> MLEEALAAIQNARDLEELKALKARYLGKKGLLTQEMKGLSALPLEERRKRGQELNAIKAALEAALEAREKALEEAALKEALERERVDVSLPGASLFSGGLHPITLMERELVEIFRALGYQAVEGPEVESEFFNFDALNIPEHHPARDMWDTFWLTGEGFRLEGPLGEEVEGRLLLRTHTSPMQVRYMVAHTPPFRIVVPGRVFRFEQTDATHEAVFHQLEGLVVGEGIAMAHLKGAIYELAQAL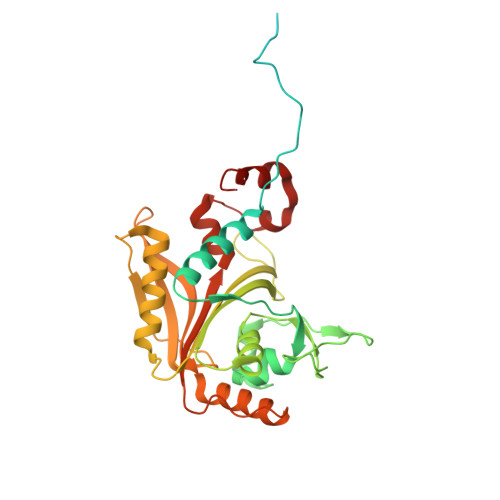FGPDSKVRFQPVYFPFVEPGAQFAVWWPEGGKWLELGGAGMVHPKVFQAVDAYRERLGLPPAYRGVTGFAFGLGVERLAMLRYGIPDIRYFFGGRLKFLEQFKGVL(2~{S})-2-(2-azanylethylamino)butanedioic acid | C6 H12 N2 O4 | 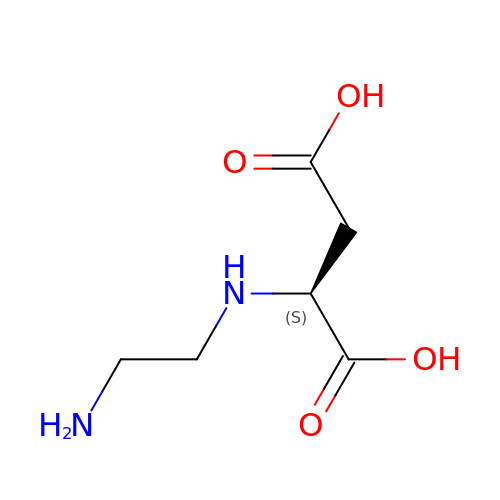PDDUTYPDHMQVSU-BYPYZUCNSA-N>GAMDPGNSAEAWYNLGNAYYKQGDYDEAIEYYQKALELDPNNAEAWYNLGNA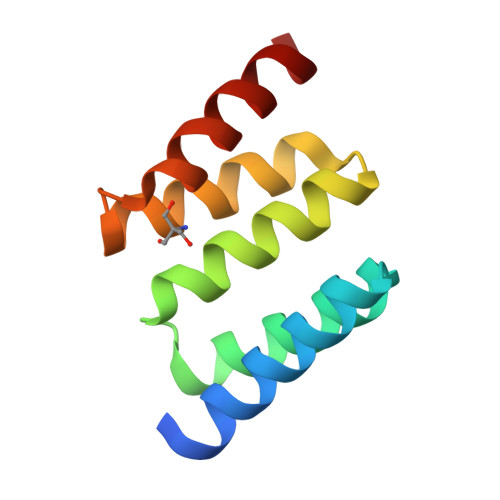YYKQGDYDEAIEYYQKALELDPNNAEAKQNLGNAKQKQG[2x]3-[2-[2-(2-azanylethoxy)ethoxy]ethoxy]propanoic acid 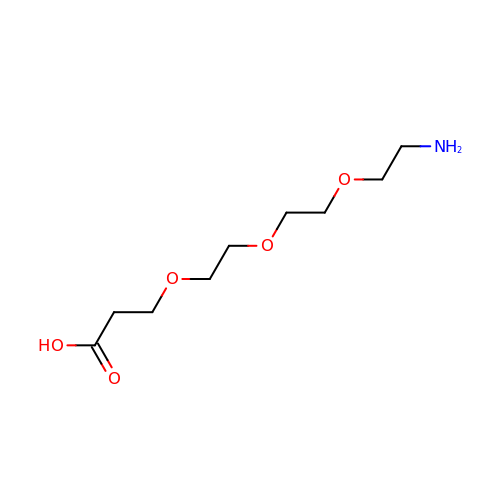| C9 H19 N O5 | XUQZKSCQPMNDEY-UHFFFAOYSA-N>GSHMNLVIALHSYEPSHDGDLGFEKGEQLRILEQSGEWWKAQSLTTGQEGFIPFNFVAKANSLEPEPWFFKNLSRKDAERQLLAPGNTHGSFLIRESESTAGSFSLSVRDFDQNQGEVVKHYKIRNLDNGGFYISPRITFPGLHELVRHYTNASDGLCT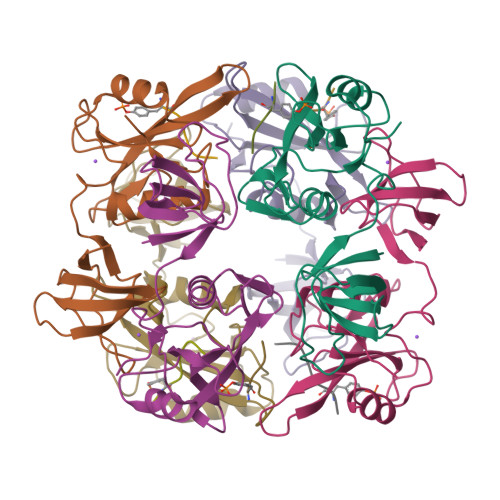RLSRPCQT[6x];>[6x]MEDYDYVHL> SLEPVYWNSANKRFQAEGGYVLYPQIGDRLDLLCPRARPPGPHSSPSYEFYKLYLVEGAQGRRCEAPPAPNLLLTCDRPDLDLRFTI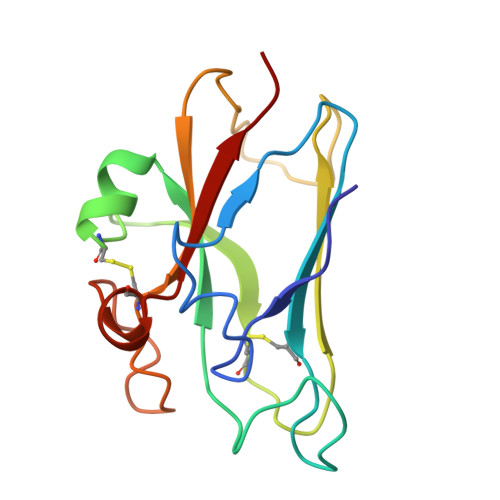KFQEYSPNLWGHEFRSHHDYYIIATSDGTREGLESLQGGVCLTRGMKVLLRVGQ>[3x]VPGPEYKVAILTVSDTVSAGAGPDRSGPRAVSVVDSSSEKLGGAKVVATAVVPDEVERIKDILQKWSD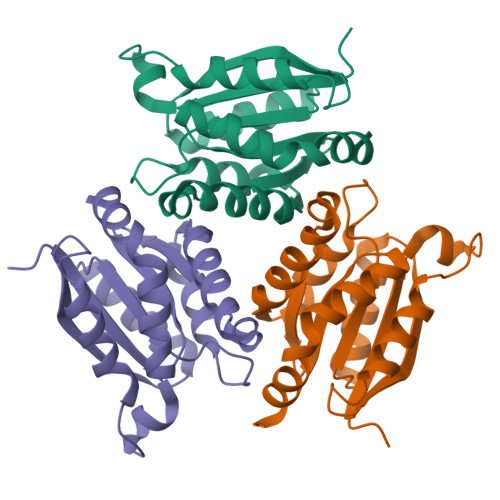VDEMDLILTLGGDGFTPRDVTPEATKKVIERETPGLLFVMMQESLKITPFAMLSRSAAGIRGSTLIINMPGNPNAVAECMEALLPALKHALKQIKGDKR>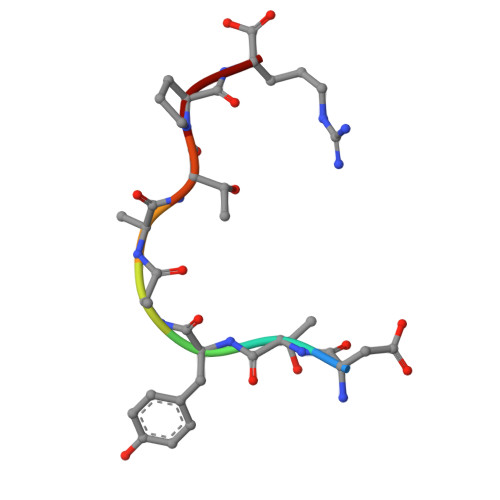 DTYAATPR> T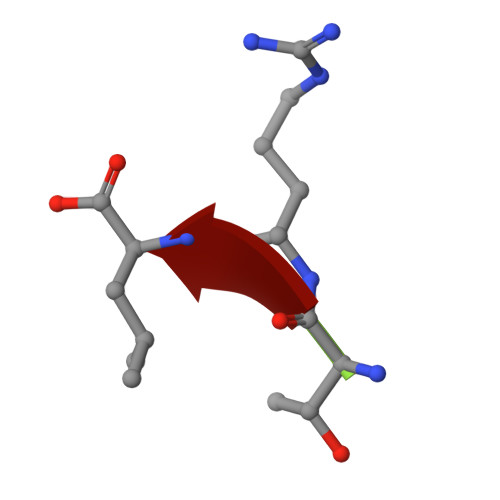RL> NQPYRTGFHFQPPKNWMNAPNGPMIYKGIYHLFYQWNPKGAVWGNIVWAHSTSTDLINWDPHPPAIFPSAPFDINGCWSGSATILPNGKPVILYTGIDPKNQQVQNIAEPKNLSDPYLREWKKSPLNPLMAPDAVNGINASSFRDPTTAWLGQDKKWRVIIGSKIHRRGLAITYTSKDFLKWEKSPEPLHYDDGSGMWECPDFFPVTRFGSNGVETSSFGEPNEILKHVLKISLDDTKHDYYTIGTYDRVKDKFVPDNGFKMDGTAPRYDYGKYYASKTFFDSAKNRRILWGWTNESSSVEDDVEKGWSGIQTIPRKIWLDRS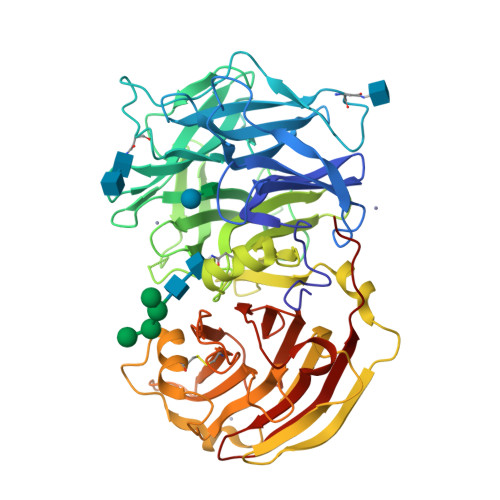GKQLIQWPVREVERLRTKQVKNLRNKVLKSGSRLEVYGVTAAQADVEVLFKVRDLEKADVIEPSWTDPQLICSKMNVSVKSGLGPFGLMVLASKNLEEYTSVYFRIFKARQNSNKYVVLMCSDQSRSSLKEDNDKTTYGAFVDINPHQPLSLRALIDHSVVESFGGKGRACITSRVYPKLAIGKSSHLFAFNYGYQSVDVLNLNAWSMNSAQIS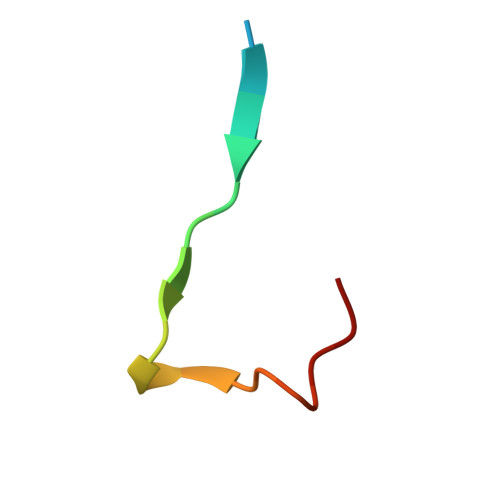> SKKVKRAKLDQTSKGPENLQFS> ENSLEIEELARFAVDEHNKKENALLEFVRVVKAKEQMHMKERQINTMYYLTLEAKDGGKKK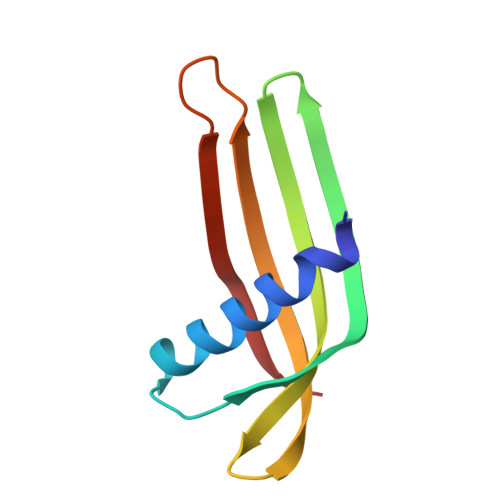LYEAKVWVKKYLGDFWKDNFKELQEFKPV> MSIQRQLTNERMSQVVVHNGTVYLAGQVGDDMTAGVEQQTREVLNSIERLLDLAGTDKTRILSVTIYLKDIDADFAGMNSVWDKWLPKGF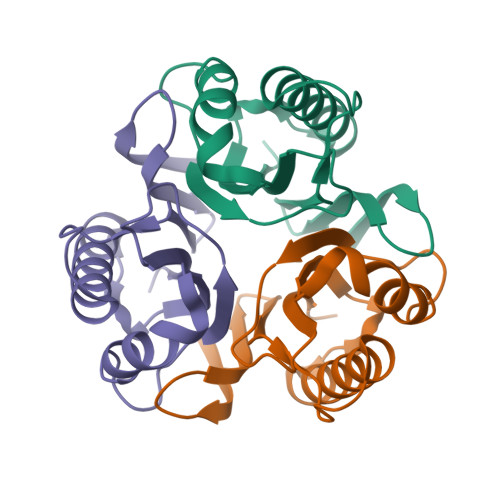APARATVEAKLCEPQILVELSVIAALP> MKVGQDKVVTIRYTLQVEGEVLDQGELSYLHGHRNLIPGLEEALEGREEGEAFQAHVPAEK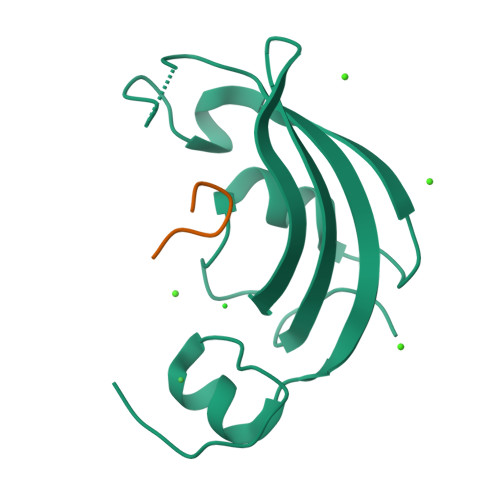AYGATGHPGIIPPHATLDFQVEVVKVREATPEELLHGHAHPSGHHHHHH;> RLGIVKPWNSTWFANX>MAQGNNYGQTSNGVADESPNMLVYRKMEDVIARMQDEKNGIPIRTVKSFLSKIPSVFSGSDIVQWLIKNLTIEDPVEALHLGTLMAAHGYFFPISDHVLTLKDDGTFYRFQTPYFWPSNCWEPENTDYAVYLCKRTMQNKARLELADYEAESLARLQRAFARKWEFIFMQAEAQAKVDKKRDKIERKILDSQERAFWDVHRPVPGCVNTTEVDIKKSSRMRNPHKTRKSVYGLQNDIRSHSPTHTPTPETKPPTEDELQQQIKYWQIQLDRHRLKMSKVADSLLSYTEQYVEYDPFLAPPDPSNPWLSDDTTFWELEASKEPSQQRVKRWGFGMDEALKDPVGREQFLKFLESEFSSENLRFWLAVEDLKKRPIREVPSRVQEIWQEFLAPGAPSAINLDSKSYDKTTQNVKEPGRYTFEDAQEHIYKLMKSDSYPRFIRSSAYQELLQAKKKGKSLTSKRLTSLVQSY[2x];>MATDGLHENETLASLKSEAESLKGKLEEERAKLHDVELHQVAERVEALGQFVMKTRRTLKGHGNKVLCMDWCKDKRRIVSSSQDGKVIVWDSFTTNKEHAVTMPCTWVMACAYAPSGCAIACGGLDNKCSVYPLTFDKNENMAAKKKSVAMHTNYLSACSFTNSDMQILTASGDGTCALWDVESGQLLQSFHGHGADVLCLDLAPSETGNTFVSGGCDKKAMVWDMRSGQCVQAFETHESDVNSVRYYPSGDAFASGSDDATCRLYDLRADREVAIYSKESIIFGASSVDFSLSGRLLFAGYNDYTINVWDVLKGSRVSILFGHENRVSTLRVSPDGTAFCSGSWDHTLRVWA[2x]

RGS proteins act as GTPase-activating proteins (GAPs) by interacting directly with activated Gα and accelerating GTP hydrolysis thereby promoting G-protein inactivation upon reassembly of the inactive Gαβγ heterotrimer. A unique hallmark of R7 RGS proteins is their modular architecture encompassing several domains and subunits. The central GGL domain forms an obligatory heterodimer with type 5 G-protein β-subunit (Gβ5) which stabilizes the complex and docks it onto effectors. RGS7 is a prototypic member of the family, broadly expressed in the nervous system and periphery and involved in regulation of multiple GPCR systems with key roles in physiology.

To gain structural insights into the specificity of the RGS7-Gβ5 interaction, we solved the 2.13 Å crystal structure of the RGS7-Gβ5 dimer complex which required buffer optimization using thermofluor. The structure contains all domains common to the R7 RGS family members: DEP-DHEX, GGL and RGS. The core of the molecule is formed by the Gβ5 subunit, which has a typical β-propeller fold commonly found in domains with WD40 repeats. Notably, Gβ5 is engulfed by all RGS7 domains, making extensive contacts at four main interfaces: the DEP domain, the DHEX-GGL linker, the Gγ-like (GGL) domain, and the RGS domain. Electron density is visible for residues 19–218 and 252–450 of chain A as well as 19–218 and 252–450 of chain B of RGS7 and for residues 2–353 of chain C and 4–353 of chain D of Gβ5. Interestingly, in RGS7, the Dα1Dα2 and Eα1Eα2 loops adopt a unique conformation in both molecules within asymmetric unit documenting yet another alternative organization and intrinsic flexibility of this region. In RGS7, the DHEX domain is lifted upward and away from Gβ5 thereby creating a wider groove between DHEX and Gβ5 when compared to RGS9. Most prominently, this includes much longer Eα1Eα2 and DEP-DHEX loops that adopt different conformations. Together, this distinct organization of the Eα1Eα2 and Dα1Dα2 loops positions them close to the invariant Eα3Eα4 loop to assemble a strong cluster of basic residues on the surface of the DEP-DHEX interface. In RGS7, the DHEX-GGL linker forms a 310-helix embedded into the β-propeller ring at the hotspot region of Gβ5. The present structure shows a unique mode of Gβ5 integration into the complex providing the first example of Gβγ like complexes in which N-terminal α-helices of both Gβ subunit and GGL are protruding away from β-propeller fold of Gβ subunit.>MQAGKPILYSYFRSSCSWRVRIALALKGIDYKTVPINLIKDRGQQFSKDFQALNPMKQVPTLKIDGITIHQSLAIIEYLEETRPTPRLLPQDPKKRASVRMISDLIAGGIQPLQNLSVLKQVGEEMQLT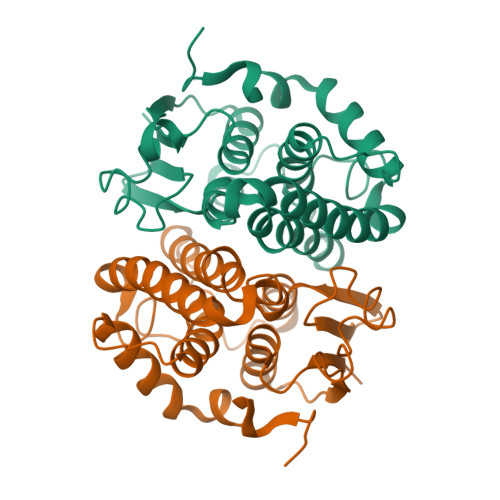WAQNAITCGFNALEQILQSTAGIYCVGDEVTMADLCLVPQVANAERFKVDLTPYPTISSINKRLLVLEAFQVSHPCRQPDTPTELRA[2x]> GSPNYDKWEMERTDITMKHKLGGGQYGEVYEGVWKKYSLTVAVKTLKEDTMEVEEFLKEAAVMKEIKHPNLVQLLGVCTREPPFYIIIEFMTYGNLLDYLRECNRQEVSAVVLLYMATQISSAMEYLEKKNFIHRDLAARNCLVGENHLVKVADFGLSRLMTGDTYTAHAGAKFPIKWTAPESLAYNKFSIKSDVWAFGVLLWEIATYGMSPYPGIDLSQVYELLEKDYRMERPEGC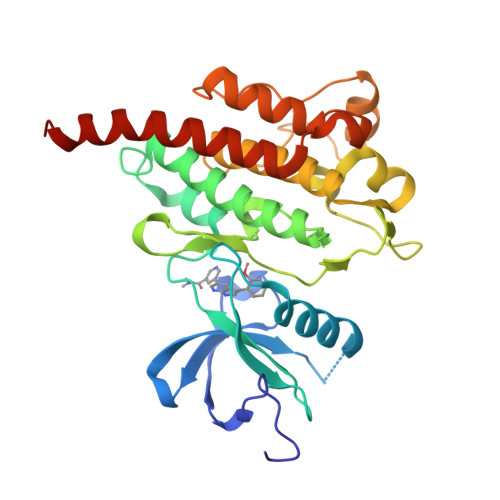PEKVYELMRACWQWNPSDRPSFAEIHQAFETMFQESSISDEVEKELGKRGT>[30x]MAQSSNSTHEPLEVLKEET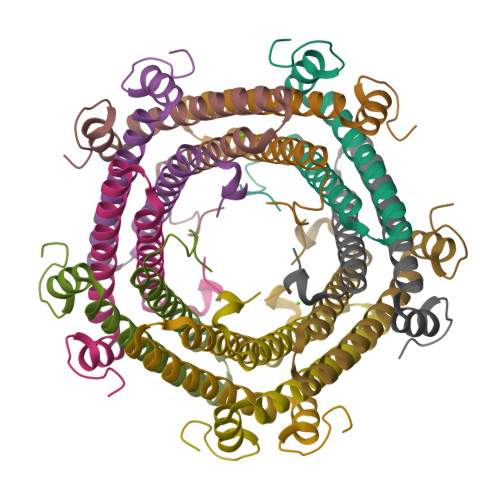VNRHRAIVSVMEALEAVDWYDQRVDASTDPELTAILAHNRDEEKEHAAMTLEWLRRNDAKWAEHLRTYLFTEGPITAANSSSVDKLAAALEHHHHHH>[2x]MTDKTLQQIDKLICSWLKQIDNVIPQLIMEMTTETKRHRFDLVTNVDKQIQQQFQQFLATYFPEHQLLAEEKSNAMITNEINHLWIMDPIDGTANLVKQQEDYCIILAYFYEGKPMLSYVYDYPHKKLYKAIRGEGAFCNGFKMEEPPSLKLEDAIISFNAQVMNLDTVQDLFDASFSYRLVGACGLDSMRVAKGQFGAHINTNPKPWDIAAQF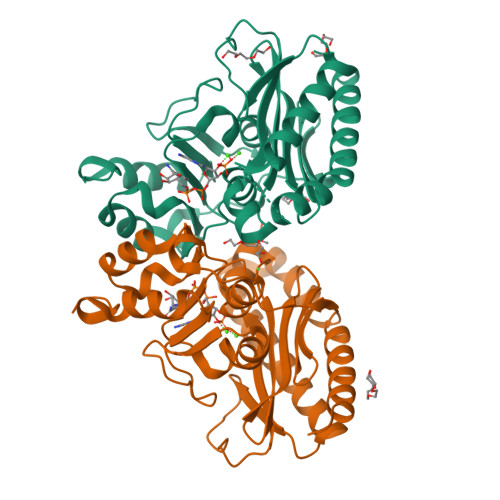LFAELLNLKMTTLDGKAIDHLKGAPFIISNKACHETVLKILNANGGYQKYR> TRPFTVPNIPLKYLSNSRIPNPIEGMSLSPDQTQNVQFQNGRCTIDGQPLGTTPVSVSQLCKFRGRITSGQRVLNLTELDGSPFMAFAAPAPAGFPDLGSCDWHIEMSKIPNS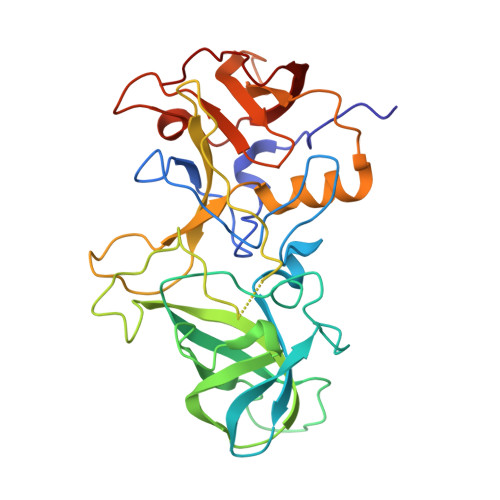STQNNPIVTNSVKPNSQQFVPHLSSITLDENVSSGGDYIGTIQWTSPPSDSGGANTNFWKIPDYGSSLAEASQLAPAVYPPGFNEVIVYFMASIPGPNQSGSPNLVPCLLPQEYITHFISEQAPIQGEAALLHYVDPDTNRNLGEFKLYPGGYLTCVPNSSSTGPQQLPLDGVFVFASWVSRFYQLKPVG>MMEYKIVENGLTYRIGNGASVPISNTGELIKGLRNYGPYEVPSLKYNQIALIHNNQFSSLINQLKSQISSKIDEVWHIHNINISEFIYDSPHFDSIKSQVDNAIDTGVDGIMLVLPEYNTPLYYKLKSYLINSIPSQFMRYDILSNRNLTFYVDNLLVQFVSKLGGKPWILNVDPEKGSDIIIGTGATRIDNVNLFCFAMVFKKDGTMLWNEISPIVTSSEYLTY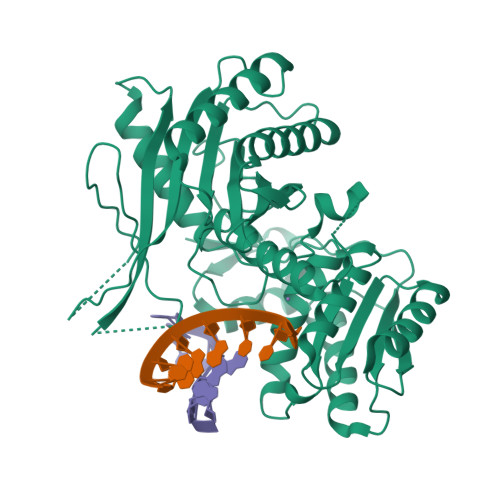LKSTIKKVVYGFKKSNPDWDVEKLTLHVSGKRPKMKDGETKILKETVEELKKQEMVSRDVKYAILHLNETHPFWVMGDPNNRFHPYEGTKVKLSSKRYLLTLLQPYLKRNGLEMVTPIKPLSVEIVSDNWTSEEYYHNVHEILDEIYYLSKMNWRGFRSRNLPVTVNYPKLVAGIIANVNRYGGYPINPEGNRSLQTNPWFL[2x]> IVGGQECKDGECPWQALL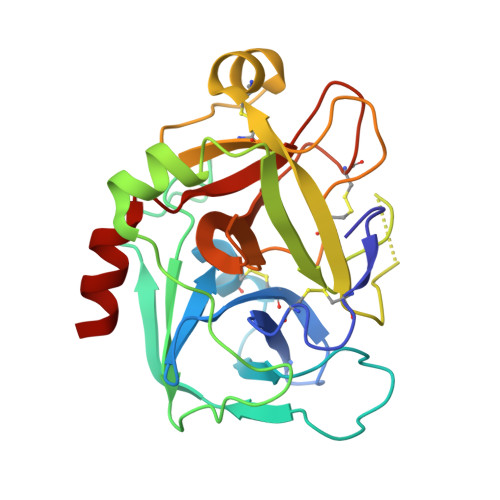INEENEGFCGGTILSEFYILTAAHCLYQAKRFKVRVGDRNTEQEEGGEAVHEVEVVIKHNRFTKETYDFDIAVLRLKTPITFRMNVAPACLPERDWAESTLMTQKTGIVSGFGRTHEKGRQSTRLKMLEVPYVDRNSCKLSSSFIITQNMFCAGYDTKQEDACQGDAGGPHVTRFKDTYFVTGIVSWGEGCARKGKYGIYTKVTAFLKWIDRSMK> MKPQKIVIKLGMPSPKNRTKAMVLAAKVYG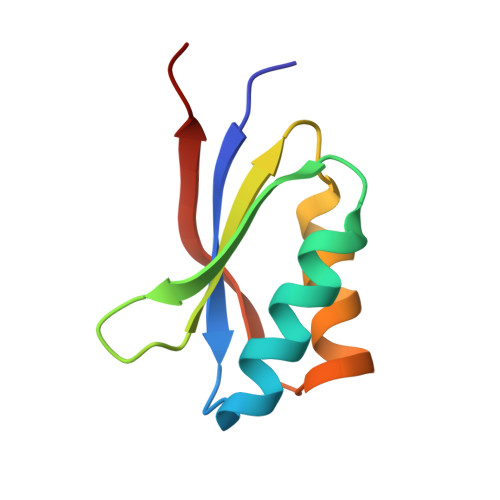VSSVAITGDDKDQLEVVGVDVDTACLVSCLRKKVLRRADIMVVEEAKDK> V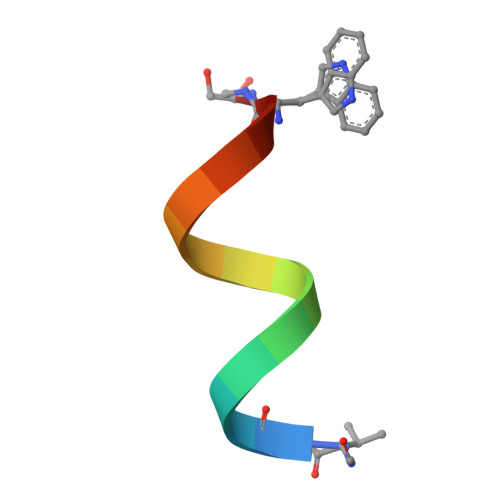GALAVVVWLFLWLWX>[3x]GEQLLKNPLIEFCDSVCRGCGQVMFQNNTVTGLLFFAGIFYNSTTLGVCAVLGTAASTLTAQLLGVDKPLVRAGLFGFNGTLA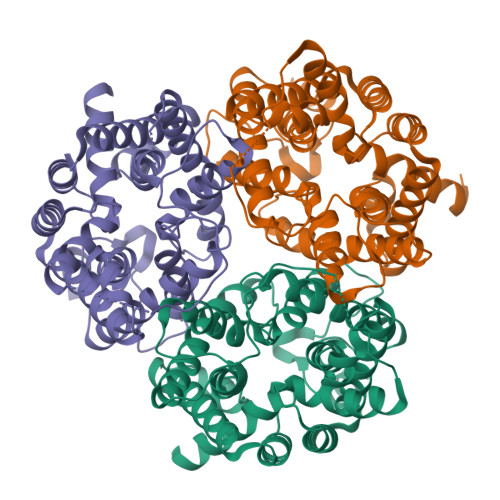GIALPFFFNYEPAMLGYVALNGAFTTIIMASLLNFLGKWGVPALTAPFVLATWLLMFGVYKLSLFHPGALIAPALPSVAGLADMGTVTGRTFMEGLFKGVGEVMFQDNIVTGVIFVVAILVNSRISALFAVIGSLVGLCTALIMHSPETPVRLGLYGFNSVLCGIAMGGIFFYLNIRTFLYALGCMVLGAIATGAFSVLLSPIGMPALTWPFIVVTWLFLFAGSMFRNIAQVPTEKAGTPEDNLRSLAIGSR> MDSKYQCVKLNDGHFMPVLGFGTYAPAEVPKSKALEATKLAIEAGFRHIDSAHLYNNEEQVGLAIRSKIADGSVKREDIFYTSKLWCNSHRPELVRPALERSLKNLQLDYVDLYLIHFPVSVKPGEEVIPKDENGKILFDTVDLC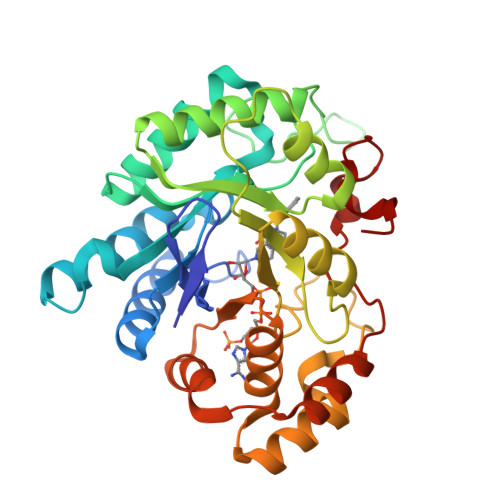ATWEAVEKCKDAGLAKSIGVSNFNRRQLEMILNKPGLKYKPVCNQVECHPYFNQRKLLDFCKSKDIVLVAYSALGSHREEPWVDPNSPVLLEDPVLCALAKKHKRTPALIALRYQLQRGVVVLAKSYNEQRIRQNVQVFEFQLTSEEMKAIDGLNRNVRYLTLDIFAGPPNYPFSDEY> A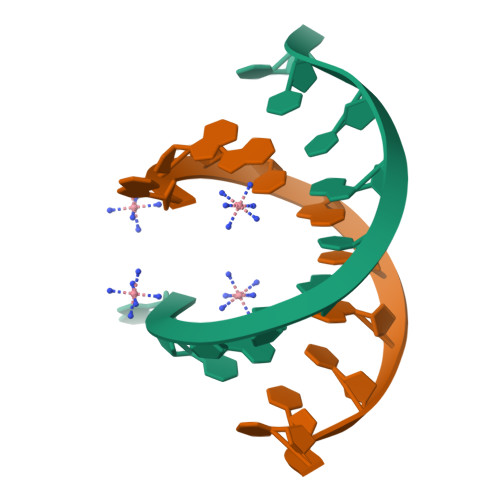GGCATGCCT> GPLGSVVRAKFNFQQTNEDELSFSKGDVIHVTRVEEGGWWEG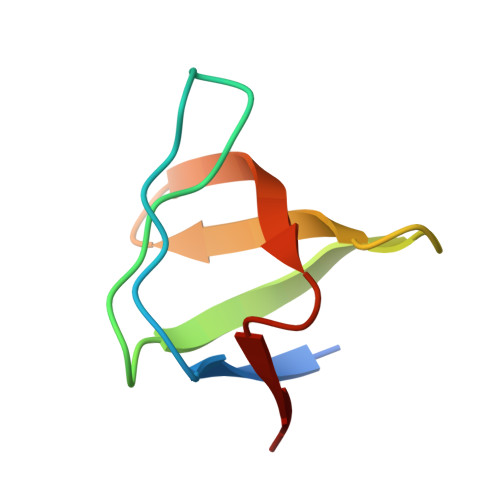THNGRTGWFPSNYVREI>MAHHHHHHMSAAALQETPSIQVKPLSAHIGAELHGVDLTRKLDPSEVAQIRAALLRWRVVFFREQFLTHEQHVAFSAQFGEPTLGHPV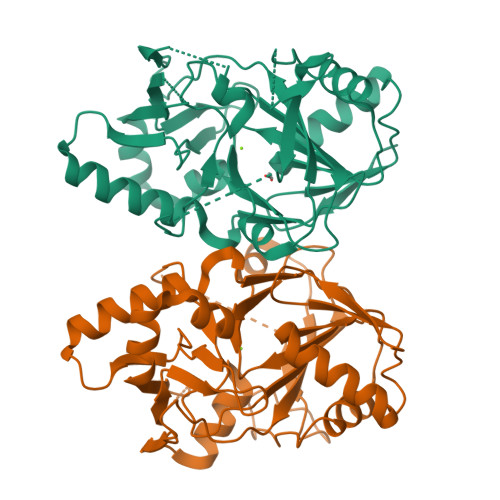FGHVDGHPEVYSISKYRKATRFEGQALLRPWTGWHTDVTAALNPPWASILRGVTIPPYGGDTQWTNLALAYEKLSAPLRAFVDGLRGVHRFTPPAGASGTEAFVKAVEQRVLVTEHPLVRVHPETGERVLYVSPSFLKSIVGVTPRESEALLELLWEHATRPEFTVRFKWEAGSVAFWDNRATAHLAPTDIFDLDFDRQLYRTTLVGDVPVGPDGRQSVAIEGSPVSAAAAVALN[2x]> AKTEPSEKSVEIMRKFSEQYARRSGTYFCVDKGVTSVVIKGLAEHKDSYGAPLCPCRHY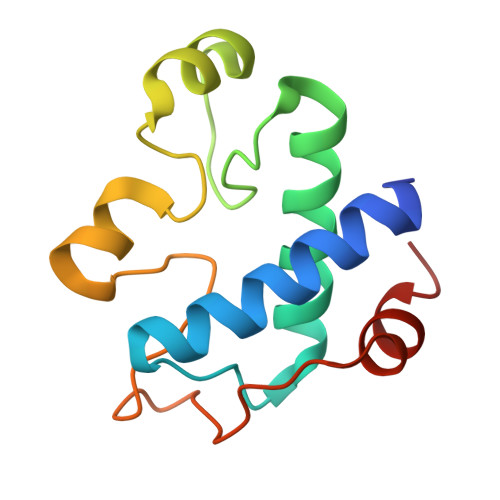DDKAAEVGQGFWNCPCVPMRERKECHCMLFLTPDNDFAGKDQTITSDEIKETTANM7-(hydroxyamino)-N-(pyridin-3-ylmethyl)-5-(trifluoromethyl)-1,3-benzothiazole-2-carboxamide 3-oxide | C15 H11 F3 N4 O3 S | 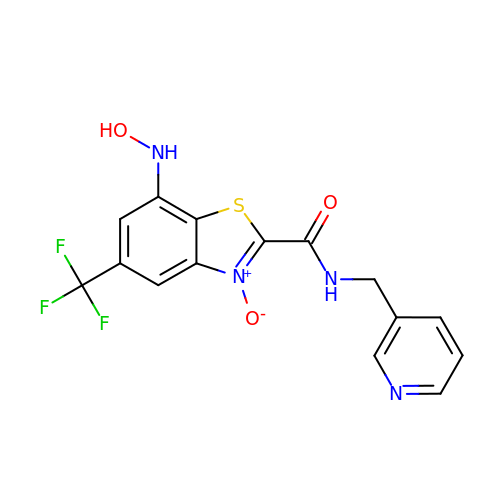GENRUIYZXCGKPM-UHFFFAOYSA-N> GPHMASMLEAKFE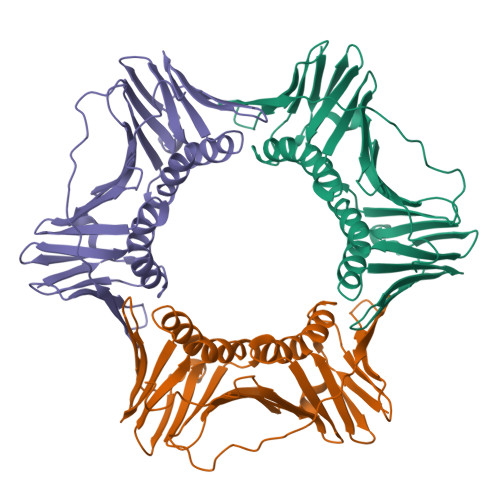EASLFKRIIDGFKKCVQLVNFQCKEDGIIAQAVDDSRVLLVSLEIGVEAFQEYRCDHPVTLGMDLTSLSKILRCGNNTDTLTLIADNTPDSIILLFEDTKKDRIAEYSLKLMDIDADFLKIEELQYDSTLSLPSSEFSKIVRDLSQLSDSINIMITKETIKFVADGDIGSGSVIIKPFVDMEHPETSIKLEMDQPVDLTFGAKYLLDIIKGSSLSDRVGIRLSSEAPALFQFDLKSGFLQFFLAPKFNDEE> 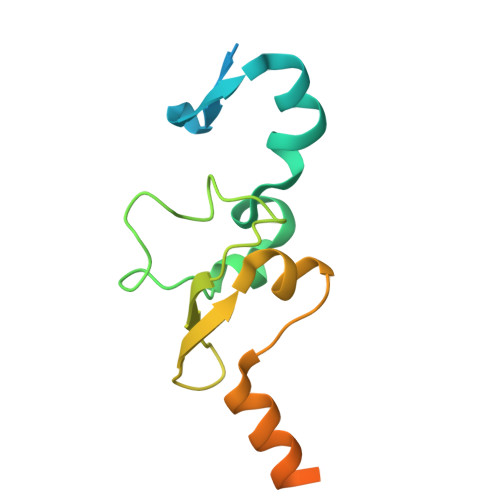MRHFGPSIAHFPLSANQLRFKASHIRIANRKRVEMFVAKRFHLPTRLATAAPDIAAEWHDELNPMHMYPAIIGIGHVQPVWWKCAICSHSYQMSVEKRVVRGGGCPQCVVNGKRAVADGALEGEMDSQLRPKRPVMFNMRTKY>MVIKPVTTPSVIQLTPDDRVTPDDKGEYQPVEKQIAGDIIRVLEFKQTNESHTGLYGIAYRAKKVIIAYALAVSGIHNVSQLPEDYYKNKDNTGRIYQEYMSNLLSALLGENGDQISKDMANDFTQNELEFGGQRLKNTWDIPDLENKLLEDYSDEDKLLALYFFASQELPMEANQQSNAANFFKVIDFLLILSAVTSLGKRIFSKNFYNGLETKSLENYIERKKLSKPFFRPPQKLPDGRTGYLAGPTKAPKLPTTSSTATTSTAASSNWRVSLQKLRDNPSRNTFMKMDDAAKRKYSSFIKEVQKGNDPRAAAASIGTKSGSNFEKLQGRDLYSIRLSQEHRVTFSINNTDQIMEIQSVGTHYQN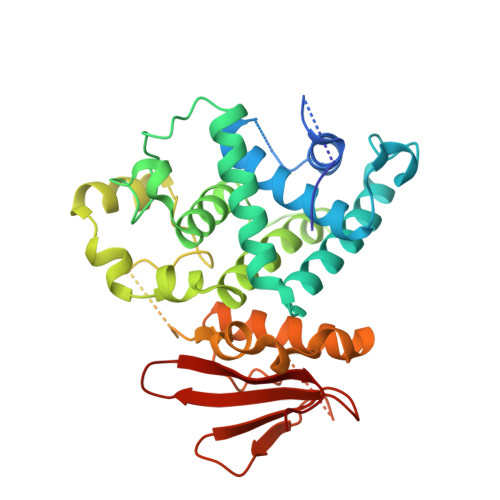I[2x]>[6x]SNAMALAAPPGELTLALTPDDKTLDPASLDRALAILAEHGILVLTGMLRTRLTDQLRTAMLDDLPEVLRQQDVPTNFVPGHVQQDPPVRESLLFPDVLLNPVVYQITHAVLGADARNAVYSGNMNLPGSHEQPVHLDEPHLWPGISHPPYCLCVDVPLIDFTLENGSTEYWPGSHVLNPDECYDERGCVLPAELERRRAVAPPVRFPIPVGSVVIRDGRL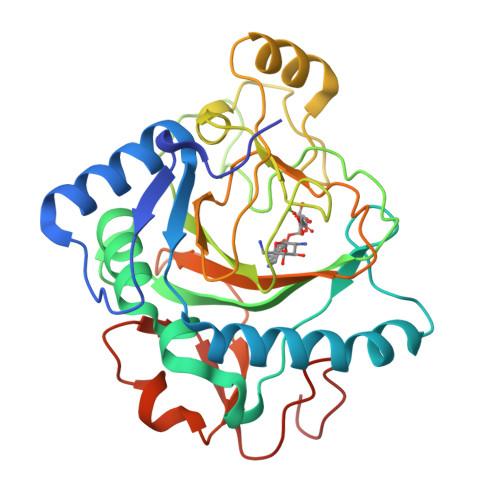WHRGVPNLSAAPRPLLAMTHYTEWFDMPPIQLPDTVKSWVDGSDRHTHAHFVAGDVDHLTGDHPFAVR>[2x]MMQGQPHQDAGMPEPYAATADVYDRLVDYAIAEWGECPRPQMADFVEQAWAARGHRV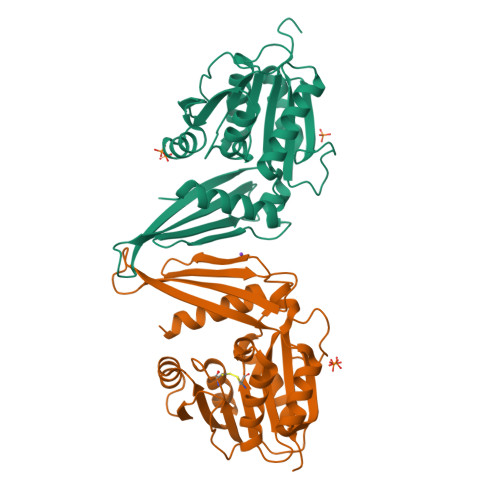RRVLELCCGTGLMTEQLVRRGYEVTAVDRSETMLALAKQRVGGAADFHQIELPAPLPDGADAVVCTAAAFNYQASARSLGETLRAVATVLPAGATFVFDIETAALLKGHWGNRVWAADEGDLAFIWDFTSEPDTTYCDVHYTQFTRHEAGADAYTGVREVHRLYAFDHDTVRAQARAAGFAQAEVFDNYTERPATDTTRYETWVLTRDERSRHHHHHH>LECYSCVQKADDGCSPNKMKTVKCAPGVDVCTEAVGAVETIHGQFSLAVRGCGSGLPGKNDRGLDLHGLLAFIQLQQCAQDRCNAKLNLTSRALDPAGNESAYPPNGVECYSCVGLSREACQGTSPPVVSCYNASDHVYKGCFDGNVTLTAANVTVSLPVRGCVQDEFC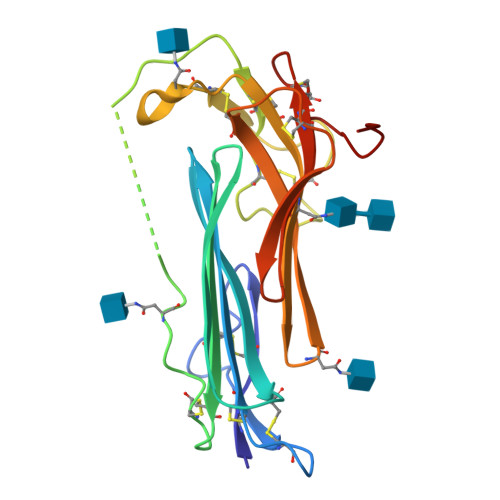TRDGVTGPGFTLSGSCCQGSRCNSDLRNKTYF[2x]>MASIEIPLHEIIRKLERMNQKKQAQRKRHKLNRKERGHKSPSEQRRSELWHARQVELSAINSDNSSDEG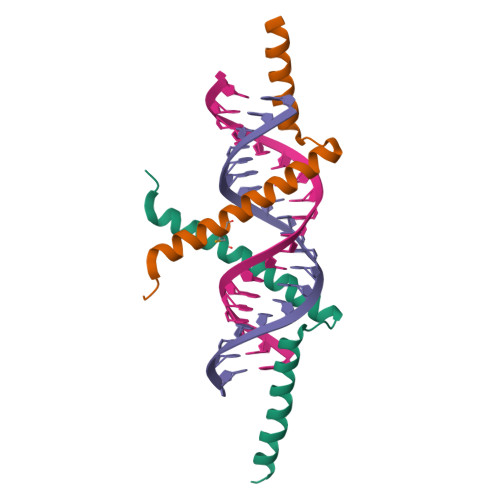HHHHHH[2x]> ESVVDLRGMWIG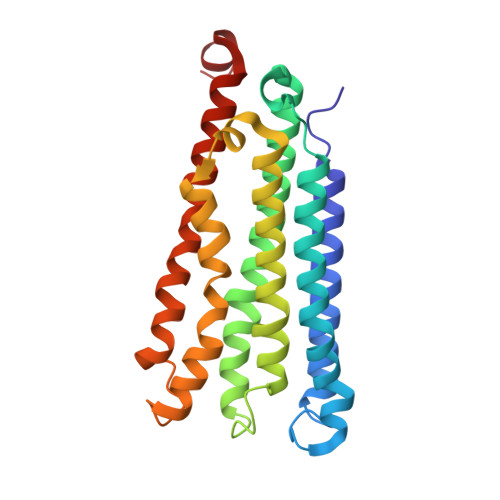LVLLNVFYLIVRIYEQVFGWRAGLDSFAPEFQTYWMSILWTEIPLELVSGLGLAGYLWKTRDRNVDAVTPREEMRRLVVLVQWLVVYGIAIYWGASFFTEQDGTWHMTVIRDTDFTPSHIIEFYMSYPIYSVIAVGAFFYAKTRIPYFAHGYSLAFLIVAIGPFMIIPNVGLNEWGHTFWFMEELFVAPLHWGFVFFGWMALGVFGVVLQILMRIHALVGKEGVKLLTE>MRSKRFEALAKRPVNQDGFVKEWIEEGFIAMESPNDPKPSIKIVNGAVTELDGKPVSDFDLIDHFIARYGINLNRAEEVMAMDSVKLANMLCDPNVKRSEIVPLTTAMTPAKIVEVVSHMNVVEMMMAMQKMRARRTPSQQAHVTNVKDNPVQIAADAAEGAWRGFDEQETTVAVARYAPFNAIALLVGSQVGRPGVLTQCSLEEATELKLGMLGHTCYAETISVYGTEPVFTDGDDTPWSKGFLASSYASRGLKMRFTSGSGSEVQMGYAEGKSMLYLEARCIYITKAAGVQGLQNGSVSCIGVPSAVPSGIRAVLAENLICSSLDLECASSNDQTFTHSDMRRTARLLMQFLPGTDFISSGYSAVPNYDNMFAGSNEDAEDFDDYNVIQRDLKVDGGLRPVREEDVIAIRNKAARALQAVFAGMGLPPITDEEVEAATYAHGSKDMPERNIVEDIKFAQEIINKNRNGLEVVKALAQGGFTDVAQDMLNIQKAKLTGDYLHTSAIIVGDGQVLSAVNDVNDYAGPATGYRLQGERWEEIKNIPGALDPNEID[2x];>[2x]MEINEKLLRQIIEDVLSEMKGSDKPVSFNAPAASAAPQATPPAGDGFLTEVGEARQGTQQDEVIIAVGPAFGLAQTVNIVGIPHKSILREVIAGIEEEGIKARVIRCFKSSDVAFVAVEGNRLSGSGISIGIQSKGTTVIHQQGLPPLSNLELFPQAPLLTLETYRQIGKNAARYAKRESPQPVPTLNDQMARPKYQAKSAILHIKETKYVVTGKNPQELRVAL;>MNTDAIESMVRDVLSRMNSLQGEAPAAAPAAGGASRSARVSDYPLANKHPEWVKTATNKTLDDFTLENVLSNKVTAQDMRITPETLRLQASIAKDAGRDRLAMNFERAAELTAVPDDRILEIYN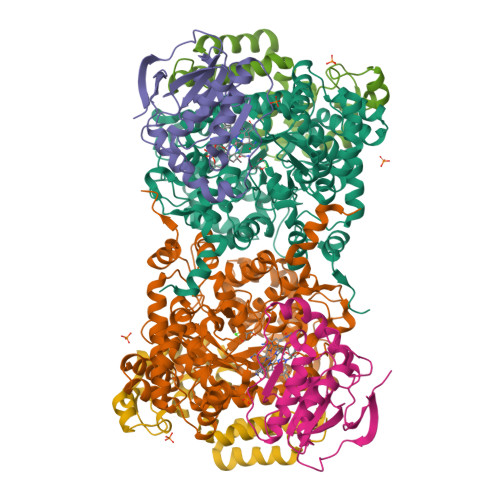ALRPYRSTKEELLAIADDLESRYQAKICAAFVREAATLYVERKKLKGDD[2x]Pseudomonas aeruginosa CtpA is a carboxyl-terminal processing protease that partners with the outer membrane lipoprotein LbcA to degrade at least five cell wall-associated proteins, four of which are cell wall hydrolases. Instead, it requires the adaptor protein LbcA, the lipoprotein-binding partner of CtpA, for activity in vivo and in vitro. Therefore, it appears that LbcA interacts with CtpA to assemble an active proteolytic complex, which controls the activity of these enzymes by degrading them. We show that CtpA alone assembles as an inactive trimer of dimers and that LbcA is a right-handed spiral that might wrap around a substrate protein.

We solved the crystal structure of CtpA that was catalytically inactive due to an S302A substitution and found that it was also in the inactive configuration. (A) overall structure of CtpA(S302A) in ribbons, with the catalytic triad residues in sticks and the point mutation S302A in red sticks. The addition of purified LbcA was able to activate the protease of wild-type CtpA but not of the mutant CtpA(S302A). For comparison, the catalytic triad Ser-309–Lys-334–Gln-338 in the protease-active B. subtilis CtpB are all within hydrogen-bonding distance. Therefore, unlike CtpB, which fluctuates between an active and inactive form in solution and can be activated by a protein substrate, the CtpA hexamer is locked in an inactive configuration and requires LbcA for activation.

>[2x]GSHMSAPLPLDELRTFAEVLDRVKAAYVEPVDDKTLLENAIKGMLSNLDPHSAYLGPEDFAELQESTSGEFGGLGIEVGSEDGFIKVVSPIDDTPAARAGIQPGDLIVQIDGKPTKGQSMTEAVDSMRGKAGSPITLTIVRDGGRPFDVELKRAIIKVKSVKSQVLEPGYAYLRITQFQVNTGEEVVKALNQLRKDNKGRLKGLVLDLRNNPGGVLQSAVEVADAFLTKGLIVYTKGRIANSELRFSADPADPSDKVPLVVLINGGSAAAAEIVAGALQDQKRAILMGTDSFGKGSVQTVLPLNNDRALKLTTALYYTPNGRSIQAQGIVPDIEVGRAKVTQERSSFEGFKEADLQGHLANGNGGADRPTGKRAAPSERPQDSDYQLSQALSLLKGLSVTRG>[2x]MTEPIFMVGARGCGKTTVGRELARALGYEFVDTDIFMQHTSGMTVADVVAAEGWPGFRRRESEALQAVATPNRVVATGG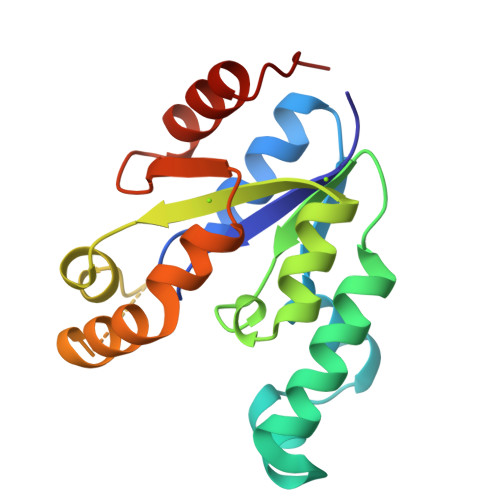GMVLLEQNRQFMRAHGTVVYLFAPAEELALRLQASPQAHQRPTLTGRPIAEEMEAVLREREALYQDVAHYVVDATQPPAAIVCELMQTMRLPAA>EENFSRSYPCDEKKQNDSVIAECSNRRLQEVPQTVGKYVTELDLSDNFITHITNESFQGLQNLTKINLNHNPNVQHQNGNPGIQSNGLNITDGAFLNLKNLRELLLEDNQLPQIPSGLPESLTELSLIQNNIYNITKEGISRLINLKNLYLAWNCYFNKVCEKTNIEDGVFETLTNLELLSLSFNSLSHVPPKLPSSLRKLFLSNTQIKYISEEDFKGLINLTLLDLSGNCPRCFNAPFPCVPCDGGASINIDRFAFQNLTQLRYLNLSSTSLRKINAAWFKNMPHLKVLDLEFNYLVGEIASGAFLTMLPRLEILDLSFNYIKGSYPQHINISRNFSKLLSLRALHLRGYVFQELREDDFQPLMQLPNLSTINLGINFIKQIDFKLFQNFSNLEIIYLSENRISPLVKDTRQSYANSSSFQRHIRKRRSTDFEFDPHSNFYHFTRPLIKPQCAAYGKALDLSLNSIFFIGPNQFENLPDIACLNLSANSNAQVLSGTEFSAIPHVKYLDLTNNRLDFDNASALTELSDLEVLDLSYNSHYFRIAGVTHHLEFIQNF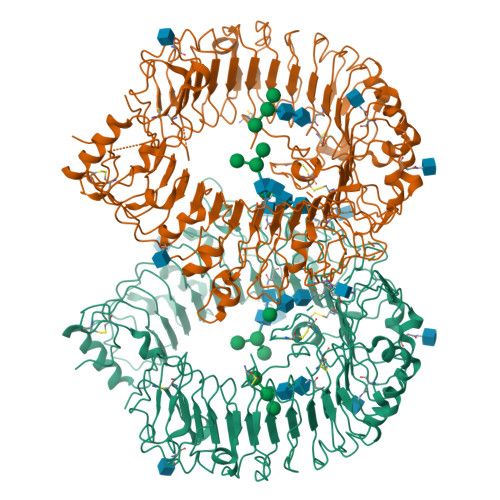TNLKVLNLSHNNIYTLTDKYNLESKSLVELVFSGNRLDILWNDDDNRYISIFKGLKNLTRLDLSLNRLKHIPNEAFLNLPASLTELHINDNMLKFFNWTLLQQFPRLELLDLRGNKLLFLTDSLSDFTSSLRTLLLSHNRISHLPSGFLSEVSSLKHLDLSSNLLKTINKSALETKTTTKLSMLELHGNPFECTCDIGDFRRWMDEHLNVKIPRLVDVICASPGDQRGKSIVSLELTTCVSDVTEFLVPR[2x]> GSKTLMGNPWFQRAKMPRALDFSGH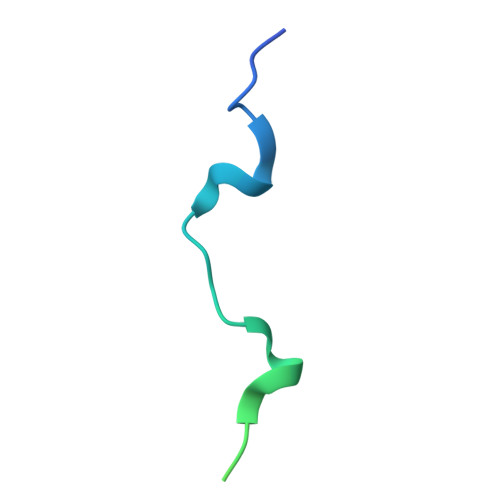THPVATFQPSRPESVNDLFLCPQKELTGNS>GSRAQSSPAAPASLSAPEPASQARVLSSSETPARTLPFTTGLIYDSVMLKHQCSCGDNSRHPEHAGRIQSIWSRLQERGLRSQCECLRGRKASLEELQSVHSERHVLLYGTNPLSRLKLDNGKLAGLLAQRMFVMLPCGGVGVDTDTIWNELHSSNAARWAAGSVTDLAFKVASRELKNGFAVVRPPGHHADHSTAMGFCFFNSVAIACRQLQQQSKASKILIVDWDVHHGNGTQQTFYQDPSVLYISLHRHDDGNFFPGSGAVDEVGAGSGEGFNVNVAWAGGLDPPMGDPEYLAAFRIVVMPIAREFSPDLVLVSAGFDAAEGHPAPLGGYHVSAKCFGYMTQQLM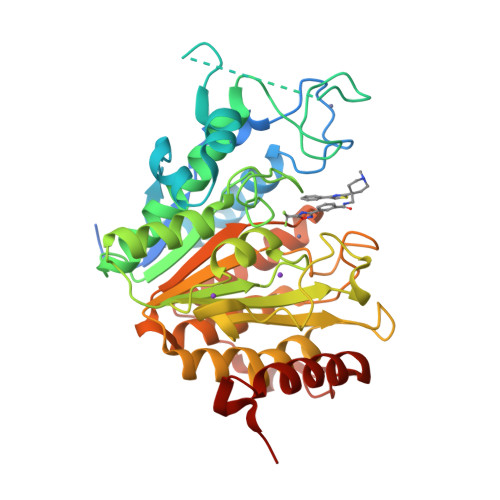NLAGGAVVLALEGGHDLTAICDASEACVAALLGNRVDPLSEEGWKQKPNLNAIRSLEAVIRVHSKYWGCMQRLAS[3x]> DPWAMTAEEKAKAVPLIHQEGNRLYREGHVKEAAAKYYDAIACLKNLQMKEQPGSPEWIQLDQQITPLLLN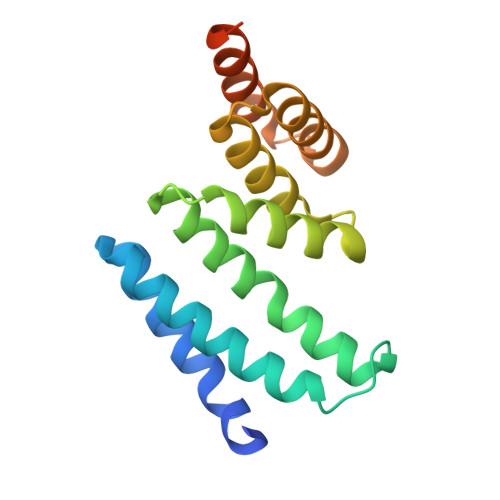YCQCKLVVEEYYEVLDHCSSILNKYDDNVKAYFKRGKAHAAVWNAQEAQADFAKVLELDPALAPVVSRELQALEARIRQKDEEDKARFRGIFSH>MKAPVRVAVTGAAGQIGYSLLFRIAAGEMLGKDQPVILQLLEIPQAMKALEGVVMELEDCAFPLLAGLEATDDPDVAFKDADYALLVGAAPRKAGMERRDLLQVNGKIFTEQGRALAEVAKKDVKVLVVGNPANTNALIAYKNAPGLNPRNFTAMTRLDHNRAKAQLAKKTGTGVDRIRRMTVWGNHSSIMFPDLFHAEVDGRPALELVDMEWYEKVFIPTVAQRGAAIIQARGASSAASAANAAIEHIRDWALGTPEGDWVSMAVPSQGEYGIPEGIVYSFPVTAKDGAYRVV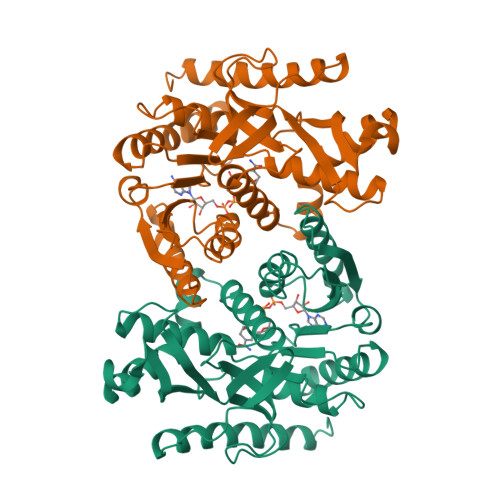EGLEINEFARKRMEITAQELLDEMEQVKALGLI[2x]>MRLRVDVIPGEHLAYPDVVLVVDVIRATTTAAAFLEAGAEALYWTPSLESALAFKDEDVVLAGETGGLKPPRFDLGNSPREALSAQVAGRVVVMSTTNGTKAAHAAARTAKHVLLASLYNAHAAARLARELATEEVA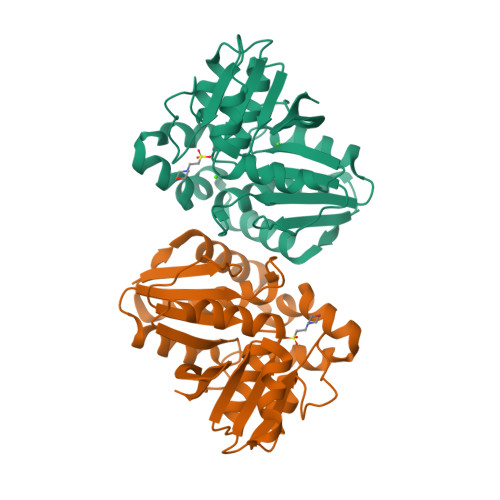ILCAGKEGRAGLDDLYTAGVLAEYLGFLGEVEPEDGARVALAVKRAYPDPLEALSLSAAALALKQVGLEADVPFCAQVAKSAAVPVLRGRVGEALIFKRA[8x]>GAMGS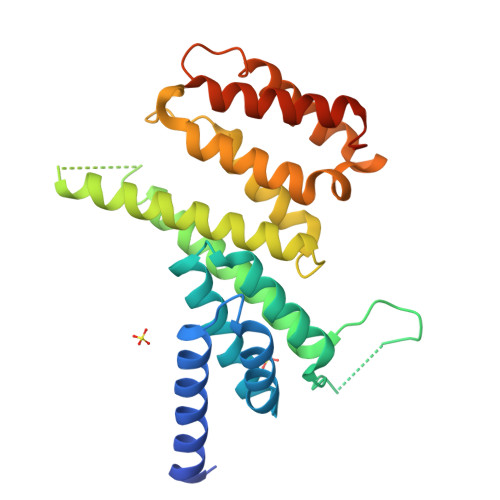NSAANNSANEKERHDAIFRKVRGILNKLTPEKFDKLCLELLNVGVESKLILKGVILLIVDKALEEPKYSSLYAQLCLRLAEDAPNFDGPAAEGQPGQKQSTTFRRLLISKLQDEFENRTRNVDVYDKRENPLLPEEEEQRAIAKIKMLGNIKFIGELGKLDLIHESILHKCIKTLLEKKKRVQLKDMGEDLECLCQIMRTVGPRLDHERAKSLMDQYFARMCSLMLSKELPARIRFLLQDTVELREHHWVPRKAFLDNGPKTI[2x]>MGSDKIHHHHHHMKIDILDKGFVELVDVMGNDLSAVRAARVSFDMGLKDEERDRHLIEYLMKHGHETPFEHIVFTFHVKAPIFVARQWFRHRIASYNELSGRYSKLSYEFYIPSPERLEGYKTTIPPERVTEKISEIVDKAYRTYLELIESGVPREVARIVLPLNLYTRFFWTVNARSLMNFLNLRADSHAQWEIQQYALAIARIFKEKCPWTFEAFLKYAYKGDILKEVQV[4x]

In prokaryotes and some archaea, the homotetrameric flavin-dependent thymidylate synthase homotetrameric ThyX catalyzes dUMP methylation into dTMP, making ThyX mandatory for cell survival in the absence of external sources of thymidylate. ThyX relies on the flavin adenine dinucleotide (FAD) as well as N5,N10-methylenetetrahydrofolate (CH2THF) as methylene donor for activity, while nicotinamide adenine dinucleotide phosphate (NADPH) acts as an electron donor. This enzyme forms a distinct class of thymidylate synthase that differs from the human thymidylate synthase TYMS or prokaryotic ThyA in terms of structure and mechanism. Combining biochemical, spectroscopic and anaerobic crystallographic analyses, we showed that formaldehyde reacts with the reduced flavin coenzyme to form a carbinolamine intermediate used by ThyX for dUMP methylation.

In addition, we attempted to study the reaction of reduced ThyX with CH2O in crystallo. For that purpose, we crystallized reduced ThyX in a glove box and then soaked the resulting crystals with CH2O in the absence of dUMP under anaerobic conditions (FADH−•CH2O). Under these conditions, we found that CH2O diffused within ThyX active site and reacted with FADH− in crystallo, thus forming a flavin carbinolamine as ascertained by the optical spectrum of (FADH−•CH2O) crystal recorded on a micro-spectrophotometer directly coupled at the X-ray beamline at the synchrotron. Structures of apo-ThyX/synthetic flavin carbinolamine and FADH−•CH2O were determined at 2.8 and 2 Å resolution, respectively. A clear additional density on FAD was observed in both structures, specifically in three out of four FAD molecules present in apo-ThyX/synthetic flavin carbinolamine and in two FAD molecules in FADH−•CH2O. This density fits with a CH2OH group attached to the N5 atom of the isoalloxazine ring and is thus attributed to the N5-C5a carbinolamine FAD adduct in both structures: in the first case, it is the synthetic compound, while in the second it is the product of the reaction between FADH− and CH2O in crystallo. The carbinolamine adduct adopts a butterfly conformation, significantly bent along its C10a–C4a axis with a dihedral angle ~12° and its N5 is pyramidal, consistent with an sp3 hybridized nitrogen and alkylation of N5. In both structures, the carbinolamine groups adopt a similar axial position lying toward the si-face of FAD and interact with a water molecule. In the case of the FADH−•CH2O structure, an inorganic phosphate occupies the dUMP-binding site and makes an additional interaction with the carbinolamine moiety. Our structures are perfectly superimposable with that of the ThyX/dUMP/folate ternary complex previously reported, with the phosphate ligand placed at a position similar to that of the phosphate group of dUMP.>MGEQNNRPTDERIIDPSTANTQLTGGVTYNTTSGGNKPLAGSPYGYETWIDTGGGVCSLTWYGADQGGGAAFKATWTNPHDFLGRLGYFWNENKPYSHYENIYCGFNYTRSGRKTAGDYSYIGIYGWSRNPSASNSNERLIEYYIVEDWFGNQWQADTSPMGINTTGGTVMGSFTVDGSSYQIIKNTRVNQPSIEGDKTFVQYFSIRQSPRKSGTISITEHFRKWERLGMKLGDNMYECKFLIEAGAGEGFFDARLIQFYRADNE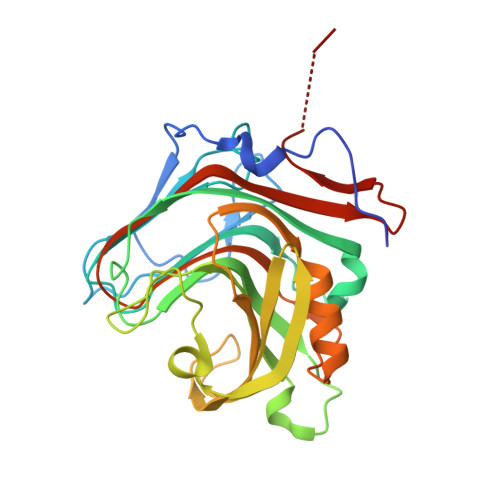GNILQITPLEHHHHHH[2x]>SMRKKIFKPEELRQALMPTLEALYRQDPESLPFRQPVDPQLLGIPDYFDIVKNPMDLSTIKRKLDTGQYQEPWQY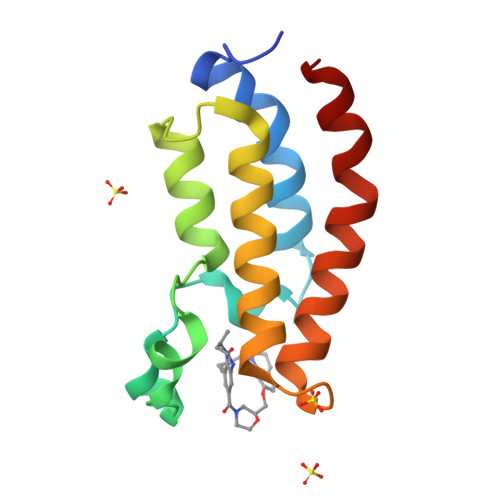VDDVWLMFNNAWLYNRKTSRVYKFCSKLAEVFEQEIDPVMQSLG[7x]>GSHMSKKGQTLMLFVGVVDPSQPDRSDIRPFTEKWTQIWQSQLYNNHVDLQVFVIDDNRAIFMFKNGEQAFEAKKFLLKQEFVSEVTIEG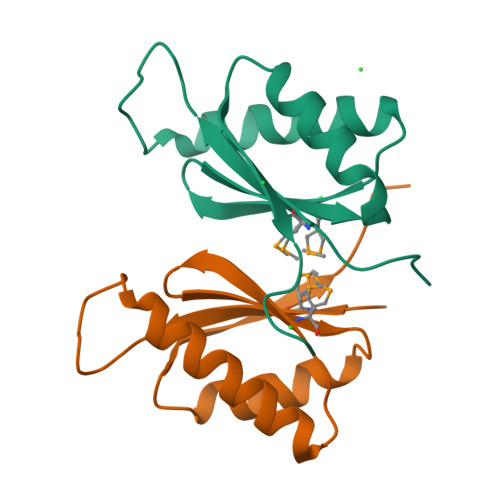QSFDG[2x]> CCTCTCGTCTCC;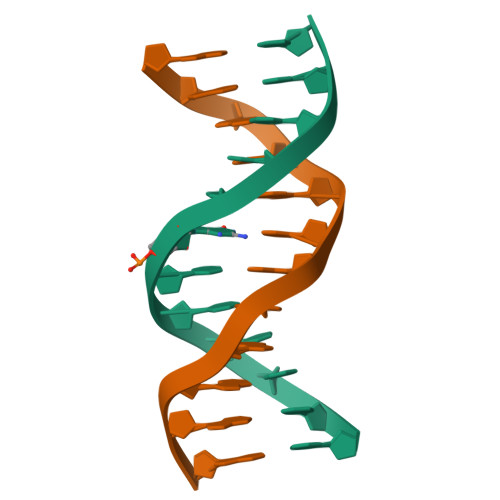> GGAGACGAGAGG>LTLWTTPDPSPNCTIDQERDSKLTLVLTKCGSQILANVSLLVVKGKFSNINNNTNPTDKKITVKLLFNEKGVLMDSSTLKKEYWNYRNDNSTVSQAYDNAVPFMPNIKAYPKPTTDTSAKPEDKKSAAKRYIVSNVYIGGLPDKTVVITIKFNAETECAYSITFEFTWAKTFEDVQFDSSSFTFSYIAQENEDEDK[6x]

Each protein forms key interactions to promote cell infection, with the terminal domain of the fiber, the fiber knob protein, interacting with the viruses’ primary cell entry receptor. The adenovirus fiber knob protein is known to have a highly conserved trimeric structure. Sialic acid (SA) usage has been proposed as a cell infection mechanism for EKC causing HAdV-D. Here we highlight an important role for SA engagement by many HAdV-D. We provide apo state crystal structures of 7 previously undetermined HAdV-D fiber-knob proteins, and structures of HAdV-D25, D29, D30 and D53 fiber-knob proteins in complex with SA. Our findings demonstrate a conserved binding site for sialic acid, common across the species D adenoviruses, therefore suggesting that, along with CAR, the receptor can be used to initiate cell entry.

We performed X-ray crystallography to generate structures of species D human adenovirus fiber knob proteins HAdV-D15, D24, D29, D30, D32 and D53 in their apo states. HAdV-D15, D24 and D32 were crystallised in only their apo states, whereas HAdV-D25, D29, D30 and D53 crystals were also soaked with sialic acid. HAdV-D24 fiber knob crystals achieved only marginal resolution, and soaking rendered them too disordered for diffraction. Non-significant changes in transduction were observed when cells were transduced with viruses with the fiber-knob proteins of HAdV-D15, D24 and D29. CAR binding was investigated for fiber knob proteins of HAdV-D24, D26 and D32, and was found to be significantly weaker interacting. The respective IC50 values were quantified as 0.02931, 0.001261 and 0.01996 µg/10e5 cells. These values represent fold changes of 162, 6 and 110 times weaker compared with the IC50 value measured for HAdV-C5 fiber knob protein.> MPFVNKQFNYKDPVNGVDIAYIKIPNAGQMQPVKAFKIHNKIWVIPERDTFTNPEEGDLNPPPEAKQVPVSYYDSTYLSTDNEKDNYLKGVTKLFERIYSTDLGRMLLTSIVRGIPFWGGSTIDTELKVIDTNCINVIQPDGSYRSEELNLVIIGPSADIIQF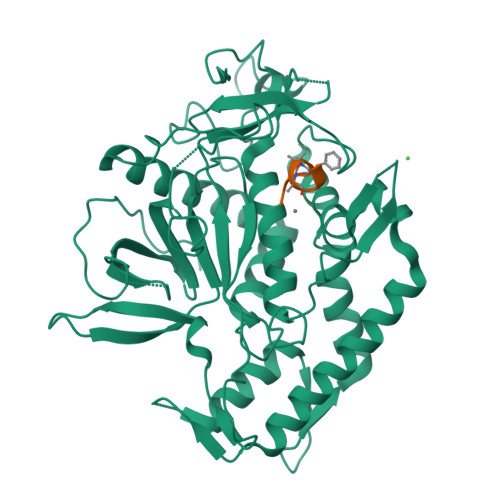ECKSFGHEVLNLTRNGYGSTQYIRFSPDFTFGFEESLEVDTNPLLGAGKFATDPAVTLAHELIHAGHRLYGIAINPNRVFKVNTNAYYEMSGLEVSFEELRTFGGHDAKFIDSLQENEFRLYYYNKFKDIASTLNKAKSIVGTTASLQYMKNVFKEKYLLSEDTSGKFSVDKLKFDKLYKMLTEIYTEDNFVKFFKVLNRKTYLNFDKAVFKINIVPKVNYTIYDGFNLRNTNLAANFNGQNTEINNMNFTKLKNFTPLVPR;> RRFAAMLA> PIFLNVLEAIEPGVVCAGHDNNQPDSFAALLSSLNELGERQLVHVVKWAKALPGFRNLHVDDQMAVIQYSWMGLMVFAMGWRSFTNVNSRMLYFAPDLVFNEYRMHKSRMYSQCVRMRHLSQEFGWLQITPQEFLCMKALLLFSIIPVDGLKNQKFFDELRMNYIKELDRIIACKRKNPTSCSRRFYQLTKLLDSVQ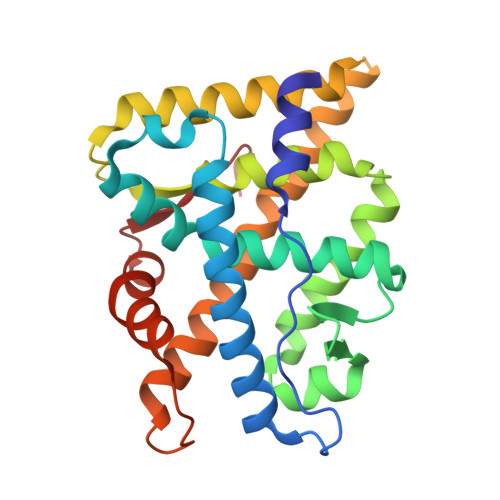PIARELHQFTFDLLIKSHMVSVDFPEMMAEIISVQVPKILSGKVKPIYFHTQ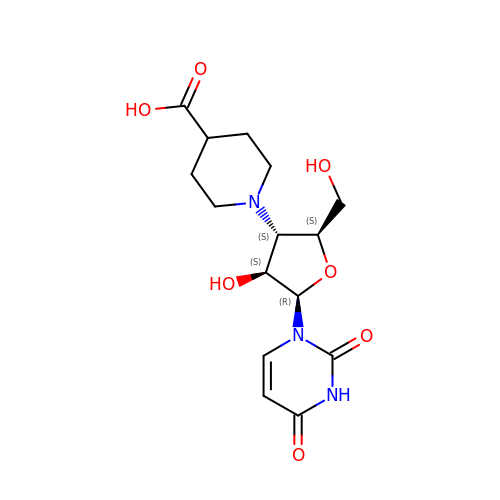1-[3-(4-CARBOXYPIPERIDIN-1-YL)-3-DEOXY-BETA-D-ARABINOFURANOSYL]PYRIMIDINE-2,4(1H,3H)-DIONE | C15 H21 N3 O7 | IBEGWFLXVPJKRI-FOUMNBMASA-N>[4x]MKAKDIVLKKSEKIEGVEVKGPWLDDAQSLEEVVSYYYRIGFQATHLGRAIEIWRKVEEKRERGEEIRVFLGYTSNIISSGLREIIAWLVKEKKVDVIVTTAGGVEEDFIKSLKPFILGDWEVDDAELRKKGVNRIGNIFVPND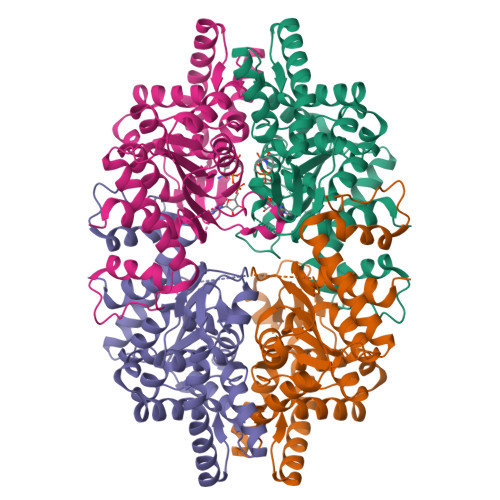RYIEFEKYMIPFFERVLKIEEKLSRPLTASEFIYEMGRYMDEKLGKEKEKSVIYWAYKNNIPIFCPAITDGSIGDMLYFFKEERRDSRLIIDIANDIVKLNNLAITAKETASIILGGSLPKHAIINANLFRGGTDYAIYISTAVPWDGSLSGAPPREGVSWGKIKAKADYVEVWGDATLIFPILVWMVMKARGQGYAQ> MKALVRLSSNHIFRSDSMSRVWLTGDAVVDLIPDGQQHYLKCPGGAPANVAVAIARLSGRSAFFGRVGNDPFGRFMQQTLTDEQVDCQHLHFDPVHRTSTVVVDLDE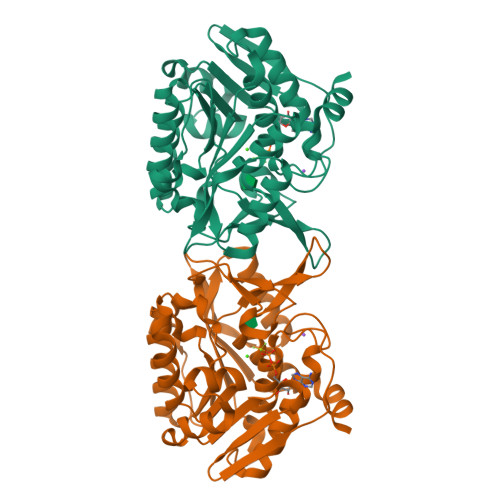HGERSFTFMVKPSADQFLQLSDIPSFQKGEWLHVCSIALANQPSRSSTFAAIAQMKEVGGYVSFDPNLREEVWSEPQELQATVMRAVGLADVVKFSEEELQFLTGTQSIEEGLQAIADFQIPLVVVTLGAKGALVATPNSQQIVSGKAVKPIDTTGAGDAFVGGLLYRLSVAQDWHNQATILDAVKWANGCGALATTQKGAMTALPNQAALYAFLE>SNAMIGKRFFQTTSKKIAFAFAIDGVLFRGKKPIAGASDALKLLNRNKIPYILLTNGGGFSERARTEFISSKLDVDVSPLQIIQSHTPYKSLVNKYSRILAVGTPSVRGVAEGYGFQDVVHQTDIVRYNRDIAPFSGLSDEQVMEYSRDIPDLTTKKFDAVLVFNDPHDWAADIQIISDAINSENGMLNTLRNEKSGKPSIPIYFSNQDLLWANPYKLNRFGQGAFRLLVRRLYLELNGEPLQDYTLGKPTKLTYDFAHHVLIDWEKRLSGKIGQSVK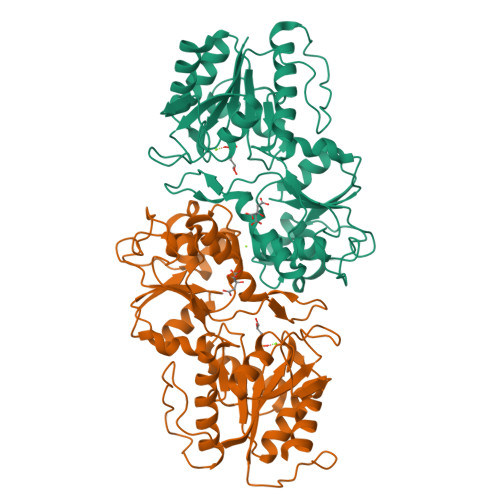QKLPLLGTKPSTSPFHAVFMVGDNPASDIIGAQNYGWNSCLVKTGVYNEGDDLKECKPTLIVNDVFDAVTKTLEKYA[2x]BLEOMYCIN A2 | C55 H85 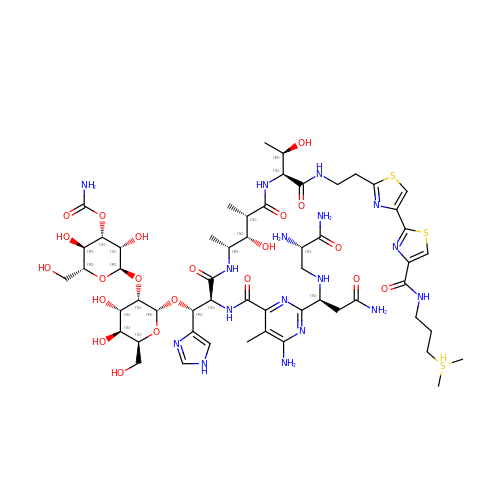N17 O21 S3 | ZGCQRJQBETWECF-UAPAGMARSA-N>[2x]MEAFEISDFKEHAKKKSMWAGALNKVTISGLMGVFTEDEDLMALPIHRDHCPALLKIFDELIVNATDHERACHSKTKKVTYIKISFDKGVFSCENDGPGIPIAKHEQASLIAKRDVYVPEVASCFFLAGTNINKAKDCIKGGTNGVGLKLAMVHSQWAILTTADGAQKYVQQINQRLDIIEPPTITPSREMFTRIELMPVYQELGYAEPLSETEQADLSAWIYLRACQCAAYVGKGTTIYYNDKPCRTGSVMALAKMYTLLSAPNSTIHTATIKADAKPYSLHPLQVAAVVSPKFKKFEHVSIINGVNCVKGEHVTFLKKTINEMVIKKFQQTIKDKNRKTTLRDSCSNIFVVIVGSIPGIEWTGQRKDELSIAENVFKTHYSIPSSFLTSMTRSIVDILLQSIS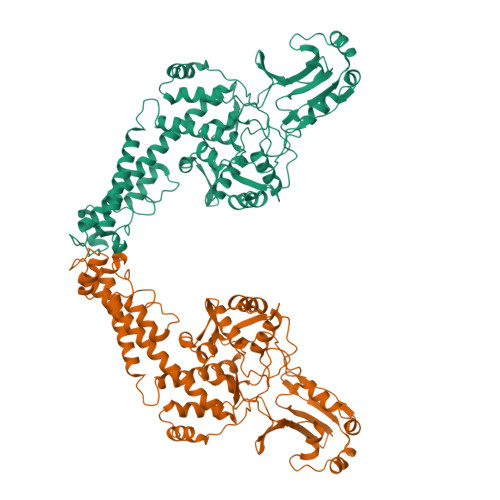KKDNHKQVDVDKYTRARNAGGKRAQDCMLLAAEGDSALSLLRTGLTLGKSNPSGPSFDFCGMISLGGVIMNACKKVTNITTDSGETIMVRNEQLTNNKVLQGIVQVLGLDFNCHYKTQEERAKLRYGCIVACVDQDLDGCGKILGLLLAYFHLFWPQLIIHGFVKRLLTPLIRVYEKGKTMPVEFYYEQEFDAWAKKQTSLVNHTVKYYKGLAAHDTHEVKSMFKHFDNMVYTFTLDDSAKELFHIYFGGESELRKRELCTGVVPLTETQTQSIHSVRRIPCSLHLQVDTKAYKLDAIERQIPNFLDGMTRARRKILAGGVKCFASNNRERKVFQFGGYVADHMFYHHGDMSLNTSIIKAAQYYPGSSHLYPVFIGIGSFGSRHLGGKDAGSPRYISVQLASEFIKTMFPAEDSWLLPYVFEDGQRAEPEYYVPVLPLAIMEYGANPSEGWKYTTWARQLEDILALVRAYVDKDNPKHELLHYAIKHKITILPLRPSNYNFKGHLKRFGQYYYSYGTYDISEQRNIITITELPLRVPTVAYIESIKKSSNRMTFIEEIIDYSSSETIEILVKLKPNSLNRIVEEFKETEEQDSIENFLRLRNCLHSHLNFVKPKGGIIEFNSYYEILYAWLPYRRELYQKRLMREHAVLKLRIIMETAIVRYINESAELNLSHYEDEKEASRILSEHGFPPLNHTLIISPEFASIEELNQKALQGCYTYILSLQARELLIAAKTRRVEKIKKMQARLDKVEQLLQESPFPGASVWLEEIDAVEKAIIKGRNTQWKFHHHHHH>MGHHHHHHGKIYSFDTLANADLIIDAVYEGGSSGNASDDPISKIIKGIGNMGGFRSAGQGIFKKLIVLYTNMEDGDWPDSIDTSKGQFIYYGDNKHPGHDIHDTPRQGNATLKMLFDSTHNEKDARRIVPPIFIFVKYPTASSSRSVQFKGVAVPGYPGLSATDDLIAVWKTTNGQRFQNYRAIFTILNIPMVSRKWINSLFDPFGQDNSLNPFYQWKISGKADVLIAPSTK[2x]

In the present study we report the crystal structure of the N-terminal DNA binding domain of the LpnPI restriction endonuclease (LpnPI-N), which recognizes the modified cytosine in the sequence context 5′-C(mC)DG-3′ (where D – A/T/G), and provide mutational/loop-swapping analysis that supports the structural model for the sequence recognition. SRA-like domains were recently identified in prokaryotes, where they serve as modules for the modified cytosine recognition by the modification-dependent restriction enzymes that protect host cells from infection by bacteriophages containing methylated, hydroxymethylated or glucosylated DNA. The modified cytosine base is extruded outside the DNA helix and accommodated in a pocket of SRA and SRA-like proteins. In summary, we show here that LpnPI recognizes the context of the flipped cytosine via several surface loops that act as separate DNA binding/recognition modules.

Here, we report the apo-structure of the DNA recognition domain of the cytosine modification-dependent restriction endonuclease LpnPI (LpnPI-N). The structure of LpnPI-N was solved at 2.1 Å resolution. The asymmetric unit contains two almost identical protein molecules (RMSD < 0.5 Å over 209 Cα atoms), with slightly larger deviations observed only at the N-termini and two flexible loops (residues 24–26 and 51–54). The largest contact surface (∼750 Å2) is formed between the N- and C-termini of both A and B subunits that encircle the 160–170 β-hairpins of the symmetry related A/B subunits. This ‘pinching’ interaction, however, is not functionally important, since LpnPI-N is a monomer in solution. The overall structure of LpnPI-N is very similar to that of the SRA-like DNA binding domain of AspBHI (RMSD 1 Å over 170 CA atoms). This allowed us to solve the LpnPI-N structure by molecular replacement using the AspBHI-N structure as an initial model. LpnPI-N is more compact than the corresponding domain of MspJI (224 versus 260 aa). The loops connecting β3–β4, β7–β8 strands and E–F helices are shorter in LpnPI-N by up to 5 aa; nevertheless LpnPI, like AspBHI, contains an 8 aa insertion in the β8 strand that breaks it into two parts.> MSGAGEALAPGPVGPQRVAEAGGGQLGSTAQGKCDKDNTEKDITQATNSHFTHGEMQDQSIWGNPSDGELIRTQPQRLPQLQTSAQVPSGEEIGKIKNGHTGLSNGNGIHHGAKHGSADNRKLSAPVSQKMHRKIQSSLSVNSDISKKSKVNAVFSQKTGSSPEDCCVHCILACLFCEFLTLCNIVL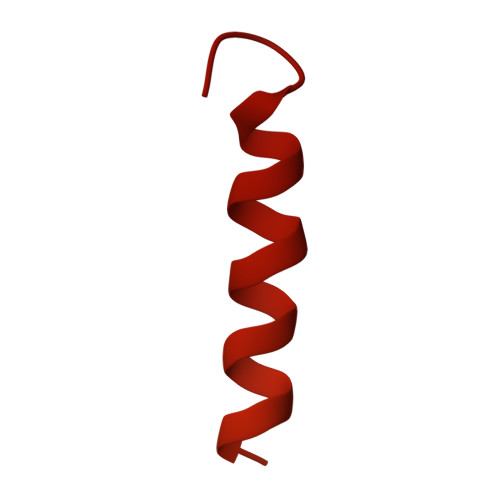GQASCGICTSEACCCCCGDEMGDDCNCPCDMDCGIMDACCESSDCLEICMECCGICFPS>[4x]PDLTAALRDVRQQYESVAAKNLQEAEEWYKSKFADLSEAANRNNDA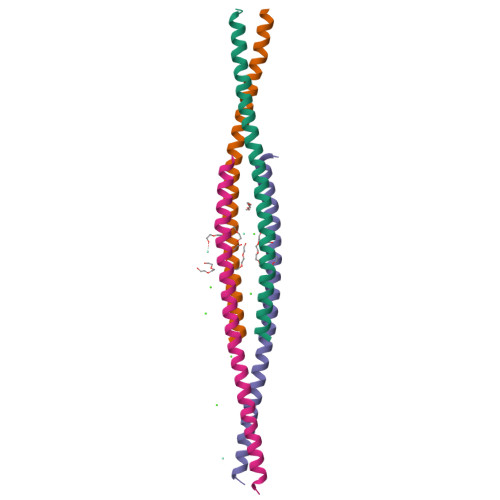LRQAKQESTEYRRQVQSLTCEVDALK> GGGUGCCAGGUAACGCCUGGGCGGGGUAACCCGACGGAAAGUGCCACAGAGAAGAGACCGCCAGCGGCCGGGGCUUCCCCCGGUGCGGGCAAGGGUGAAACGGCGGGGUAAGAGCCCACCGCCU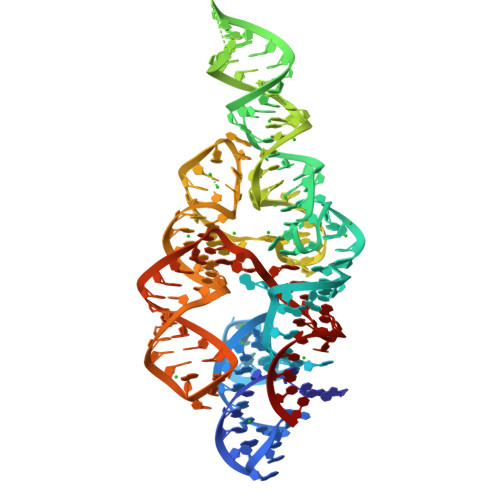GGCCUGGCAACAGGCCGGGGCACGGCAAACCCCACCC4-[(4~{S})-5-(5-chloranyl-2-oxidanylidene-1~{H}-pyridin-3-yl)-2-[2-(dimethylamino)-4-methoxy-pyrimidin-5-yl]-6-oxidanylidene-3-propan-2-yl-4~{H}-pyrrolo[3,4-c]pyrazol-4-yl]benzenecarbonitrile 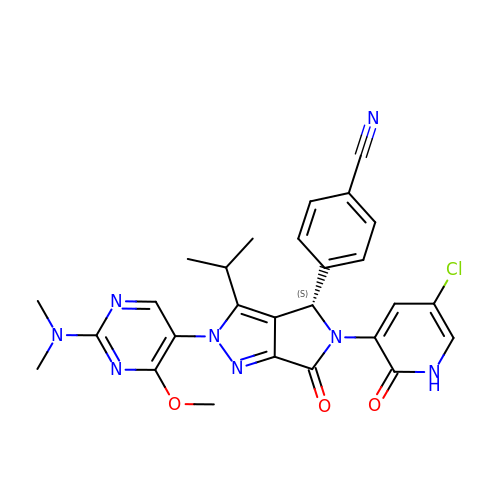| C27 H25 Cl N8 O3 | VFMRTUQQYDQOGC-QHCPKHFHSA-N>KTVRYRTYEEDEPGTVIGTLAEDLHLEGEGSFRLMKQFNNSLIHVRESDGQLSIGERIDRERICRQSPHCTLALDVVSVAKEQFKLIHVEVEVRDINDNSPRFPGAEIPVEVSESAPVGTRIPLDIATDEDVGVNSIQSFQISENSHFSIDVQTRADGVKYADLVLMKELDRESQSAYTLELLAMDGGSPSRSGTTMVNVRVLDFNDNSPVFERSSVMVELMEDAPVGHLLLDLDALDPDEGANGEIVYGFSPQVPQEVRQLFKIDAKSGRLTLEGQVDFETKQTYEFDAQAQDMALNPLTATCKVIVRVIDVNDNAPVIGITPLTSISAGVAYITEAAARESFVALISTTDRDSGQNGQVHCTLYGHEHFRLQQAYEDSYMIVTTSALDREKIAEYNLTVVAEDLGSPPFKTVKQYTIRVSDENDNAPVFAKPVYEVSVLENNAPGAYITTVVARDPDFGHNGKVIYRLVETEVMGAPITTYVSLDPATGAVYALRTFNHEILQQLDLRIQASDGGSPQLTSSAIIKVKIVDQNDNAPVIVQPALSNGSAEVVVPSRAPHGFLVTHIKAKDADEGVNAELTYSIADEGRNVFTINKATGEVFLVADVSEAI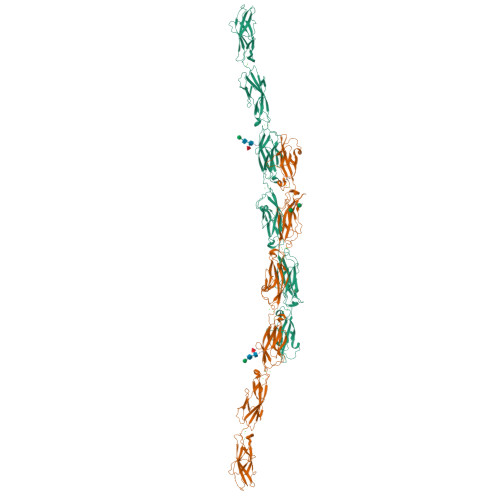GQVFRATVSVSDSGRPPLSSTATITFLVTHHHHHH[2x]>SMQLNQYKLQSEIGKGAYGVVRLAYNESEDRHYAMKVLSKKKLLKQYGFPRRPPPRGSQAAQGGPAKQLLPLERVYQEIAILKKLDHVNVVKLIEVLDDPAEDNLYLVFDLLRKGPVMEVPCDKPFSEEQARLYLRDVILGLEYLHCQKIVHRDIKPSNLLLGDDGHVKIADFGVSNQFEGNDAQLSSTAGTPAFMAPEAISDSGQSFSGKALDVWATGVTLYCFVYGKCPFIDDFILALHRKIKNEPVVFPEEPEI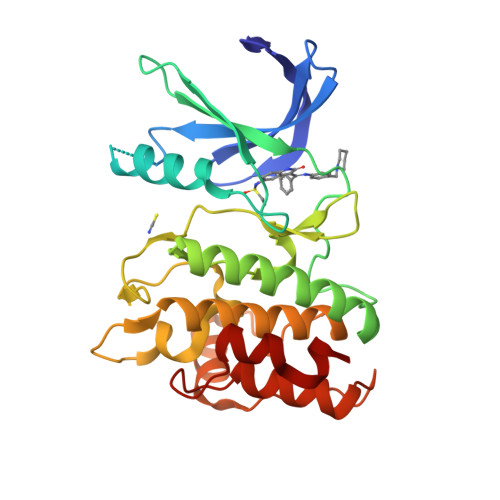SEELKDLILKMLDKNPETRIGVPDIKLHPWVTK[2x]>HHMSAIKPDMKINLRMEGNVNGHHFVIDGDGTGKPFEGKQSMDLEVKEGGPLPFAFDILTTAFHYGNRVFAEYPDHIQDYFKQSFPKGYSWERSLTFEDGGICIARNDITMEGDTFYNKVRFHGVNFPANGPVMQKKTLKWEPSTEKMYVRDG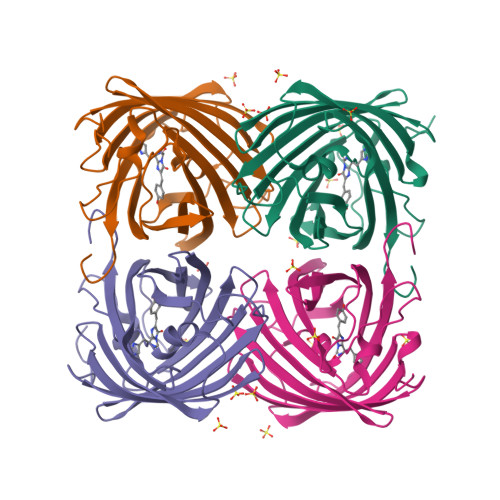VLTGDITMALLLEGNAHYRCDSRTTYKAKEKGVKLPGYHLVDHCIEILSHDKDYNKVKLYEHAVAHSGLPDN[4x]> SMGIVEEAHNLRVVGEGKRGVIVLAHGFGTDQSVWKHLVPHLVADYRVVLFDTMGAGPTNPDYFDFSRYATLEGYALDLLAILQELRVASCIYVGHSVSAVIGAIASISRPDLFSKLVLLSASPRYLNDVDYYGGFEQEDLDELFEAMGSNYKAWCSGFAPLCVGGDMESVAVQEFSRTLFNIRPDIALSVAQTIFQSDVRSLLPLVTVPCHIVQSTKDLAVPVVVSEYLHKHLGGDSIVEVMPSEGHLPQLSSPDIVIPVLLRHIQHDIAV

KAI2 receptors, classified as plant α/β hydrolase enzymes, are capable of perceiving smoke-derived butenolide signals and endogenous yet unidentified KAI2-ligands (KLs). The KAI2-mediated signaling pathway shows homology to another phytohormone signaling pathway, strigolactone (SL), where key proteins involved in KAR signaling (KAI2, D3/MAX2, and SMAX1/2) share sequence and structural similarities with proteins in the SL signaling pathway. The SL signaling pathway comprises a homologous receptor to KAI2, D14 (DWARF14), the D3/MAX2 E3 ligase, and a homologous substrate SMAX1-LIKE 6, 7, and 8 (SMXL) in Arabidopsis or D53 (DWARF53) in rice. When focusing on the binding pocket, several residues including the Ser-His-Asp catalytic triad are conserved in all proteins, highlighting its importance in the catalytic mode of action performed by α/β hydrolases.

Rice, a significant crop and representative of grasses, relies on KAI2-mediated Arbuscular mycorrhiza (AM) symbioses to flourish in traditionally arid and nutrient-poor environments. This study presents the first crystal structure of an active rice (Oryza sativa, Os) KAI2 hydrolase receptor. As observed in previously determined KAI2 crystal structures, OsKAI2 comprises of a canonical α/β-hydrolase fold with the binding pocket situated within the central core domain, beneath the helical lid domain (residues Tyr125-Ser197). Upon a closer inspection of the binding pocket, the conserved Ser-His-Asp catalytic triad is positioned at the base of the active site. The pocket comprises a hydrophobic cleft made up of phenylalanine, isoleucine, and valine residues, making it well-suited to bind the aromatic rings of KAR or KL-type ligands. The OsKAI2 pocket was compared against that of AtKAI2 (48) which shows similar pocket residues, with the exceptions of C162 and A191 in OsKAI2, which represent smaller side-chain groups in the positions of A161 and G191 in AtKAI2. The OsKAI2 pocket analyses revealed a pocket measured to have a volume of 108 Å. This is an intermediate pocket size when compared to others in the family, such as AtKAI2 with an approximate volume of 63 Å, OsD14 at 149 Å, and ShHTL7 (51) at 215 Å. Strikingly, due to its distinct proximity to the ligand binding pocket, residue C162 was selected for further inspection. Interestingly, grass KAI2s contain a cysteine at this site, resulting in a receptor that is sensitive to both (−)-GR24 and dYLG ligands. Therefore, the C162 found in grasses may be important for selectively sensing grass-related KLs or grass-related KL AM signals in the soil.>GSHMSEALKILNN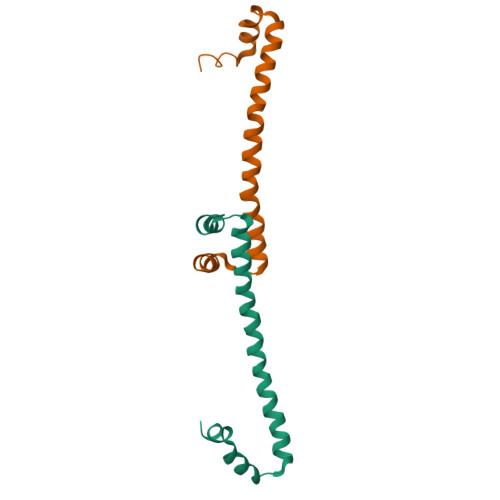IRTLRAQARESTLETLEEMLEKLEVVVNERREEESAAAAEVEERTRKLQQYREMLIADGIDPNELLNSMAAAK[2x]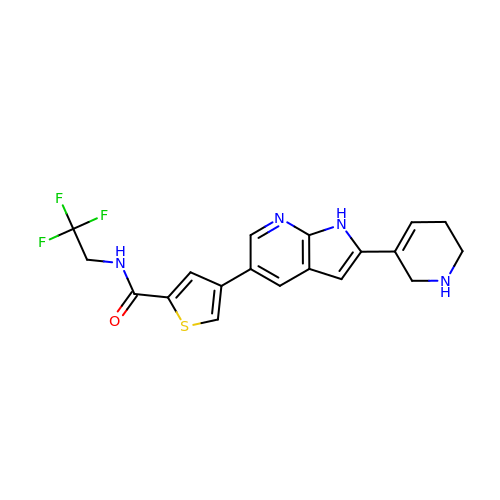(4P)-4-[(2P)-2-(1,2,5,6-tetrahydropyridin-3-yl)-1H-pyrrolo[2,3-b]pyridin-5-yl]-N-(2,2,2-trifluoroethyl)thiophene-2-carboxamide | C19 H17 F3 N4 O S | BEWNDCDAXDFYBH-UHFFFAOYSA-N(4~{S},5~{R},6~{R})-5-acetamido-6-[(1~{R},2~{S})-3-[[1-(2-ethoxyethyl)-1,2,3-triazol-4-yl]methylsulfanyl]-1,2-bis(oxidanyl)propyl]-4-oxidanyl-oxane-2-carboxylic acid | C18 H30 N4 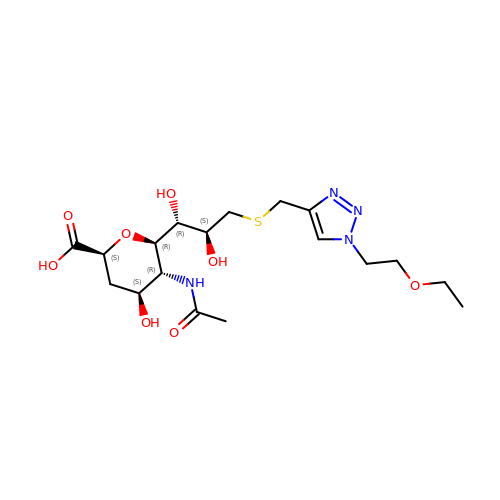O8 S | AQJNARPQFNBHOK-KMIMBKNBSA-N>MGSSHHHHHHSSGLVPRGSTSEVIEDEKQFYSKAKTYWKQIPPTVDGMLGGYGHISSIDINSSRKFLQRFLREG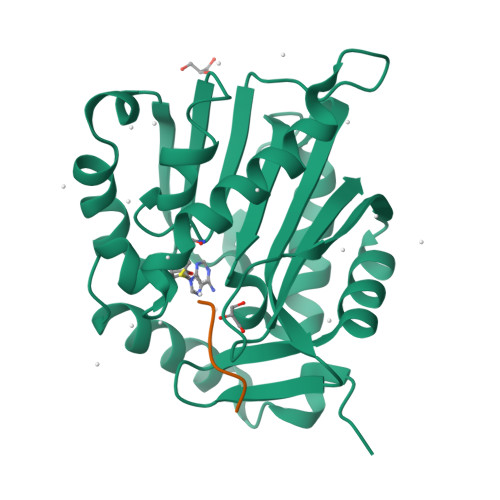PNKTGTSCALDCGAGIGRITKRLLLPLFREVDMVDITEDFLVQAKTYLGEEGKRVRNYFCCGLQDFTPEPDSYDVIWIQWVIGHLTDQHLAEFLRRCKGSLRPNGIIVIKDNMAQEGVILDDVDSSVCRDLDVVRRIICSAGLSLLAEERQENLPDEIYHVYSFALR[2x];>PPKRIA[2x]> MVRVGMRAAPRVSLEALKAALGGLKLSEAKVYLITDWQDKRDQARYALLLHTGKKDLLVPDAFGPAFPGGEEALSELVGL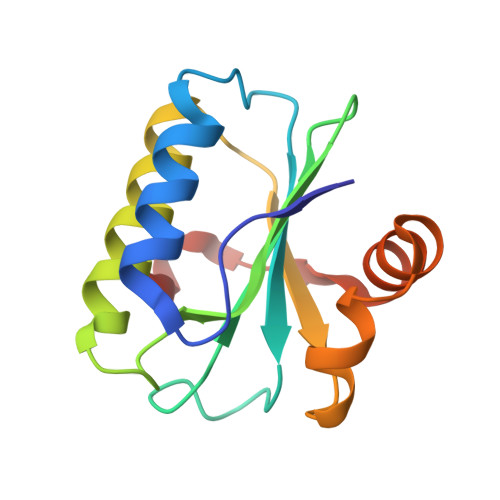LLAQGARRFYEAVVSPGEMTALLDLPPEELLKRVMAIANPTDPGIYLKRAA> GPLGSKKR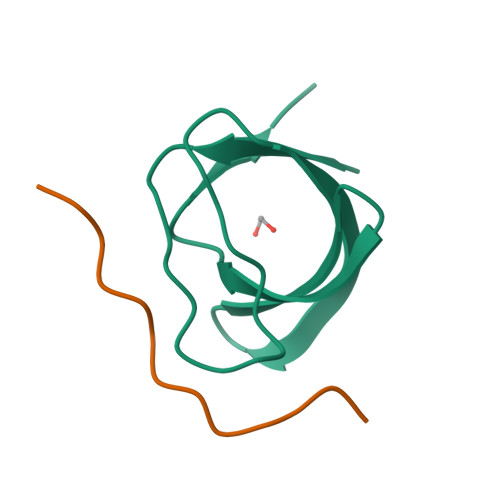QCKVLFEYIPQNEDELELKVGDIIDINEEVEEGWWSGTLNNKLGLFPSNFVKELEVT;> TAKQPPVPPPRKKRISX> GPGSEFRPQPLPPGWERRVDDRRRVYYVDHNTRTTTWQRPTMESVRNFEQWQSQRNQLQGAMQQFNQRYLYSASMLAAENDPYGPLPPGWEKRVDSTDRVYFVNHNTKTTQWEDPRTQGLQNEEPLPEGWEIRYTREGVRYFVDHNTRTTTFKDPRNGKSSVTKGGPQIAYERGFRWKLAHFRYLCQSNALPSHVKINVSRQTLFEDSFQQIMALKPYDLRRRLYVIFRGEEGLDYGGLAREWFFLLSHEVLNPMYCLFEYAGKNNYCLQINPASTINPDHLSYFCFIGRFIAMALFHGKFIDTGFSLPFYKRMLSKKLTIKDLESIDTEFYNSLIWIRDNNIEECGLEMYFSVDMEILGKVTSHDLKLGGSNILVTEENKDEYIGLMTEWRFSRGVQEQTKAFLDGFNEVVPLQWLQYFDEKELEVMLCGMQEVDLADWQRNTVYRHYTRNSKQIIWFWQFVKETDNEVRMRLLQFVTGTCRLPLGGFAELMGSNGPQKFCIEKVGKDTWLPRSHTCFNRLDLPPYKSYEQLKEKLLFAIEETEGFGQE

The Nedd4 family E3s have nine members in humans (WWP1/2, Nedd4/4 L, Smurf1/2, NEDL1/2, and Itch), which share a common N-terminal domain architecture comprised of a C2 domain and 2–4 WW domains that are responsible for subcellular localization and substrate recognition, respectively. Each HECT-type E3 contains a characteristic HECT domain at its C terminus, which catalyzes the transfer of ubiquitin from E2 to itself and then to the specific substrate. The HECT domain adopts a bilobal structure, in which the E2-binding N-lobe is connected by a flexible hinge loop to the catalytic C-lobe. To prevent excessive ubiquitination of targets and self-destruction by autoubiquitination, HECT-type E3s normally adopt an inactive state characterized by intra- or inter-molecular interaction.

To elucidate the molecular mechanism governing WWP1 autoinhibition, we determined the crystal structures of WWP1 in its fully inactive (2L34HECT) and partially active (L34HECT) states at resolutions of 2.3 Å and 2.5 Å, respectively. In the 2L34HECT crystal structure, WW2, WW4, HECT, and half of L (aa 413–427 and 432–446) are well-resolved, whereas the WW3 domain could not be modeled due to its poor electron density. The HECT domain in the closed form of WWP1 adopts a T-shape conformation, which is highly similar to that of the isolated WWP1 HECT domain structure. WW2, L, and WW4 are organized into a headset architecture, with the WW2 and WW4 domains acting as the “right ear” (denoted as “Re”) and the “left ear” (denoted as “Le”), respectively, when binding to bilateral sites of the N-lobe, whereas L functions as the “headband” of the headset (denoted as “H”) by forming a kinked α-helix that is tucked into the cleft between the N- and C-lobes of HECT. Detailed analysis of 2L34HECT suggested that the intramolecular packing is mainly driven by extensive hydrophobic and hydrogen bonding interactions. The hydrophobic Met627HECT interacts with a hydrophobic cluster formed by Trp387WW2 and Phe420L. Pro651HECT inserts into a small pocket formed by Trp409WW2 and Arg396WW2. These two core hydrophobic interactions physically anchor WW2 to HECT at the “Re” site. Hydrophobic Met434L, Phe437L, Tyr441L, and Tyr443L interact with a hydrophobic cleft formed by Phe617HECT, Phe673HECT, and Met804HECT at the “H” site, whereas, at the “Le” site, the main force driving the WW4-HECT interaction is hydrogen bonding between His517WW4 and Tyr543 in the N-terminal extension of HECT. Unexpectedly, the “IxY543”-motif in the N-terminal extension of HECT occupied the canonical “NPxY”-motif binding site in WW4.>MEVPEIEKQIGINLYSTDTTGLGGQLRQEIEDFIVKEITNREEGEEGKYLIVELTKRDWDTHHLTRTLSRILQVSQKRISVAGTKDKRALTTQKISIFDTDASEIEKIHLKDIELKVLGRSRKSVELGDLWGNDFRITVRNIENSPEETEALLKKTTDEILAQGGVPNFFGIQRFGSVRPVTHLVGKAIVEGNFEKAALLYIAEPFPEEPEETKNARQFVKDTLDFKEGLKTYPLRLGHERAMMNHLIANPEDYSGSFRVLPQNLYRMFVHGYQSYIYNIILCRRIEAGIPLNRAVEGDIVCFRNEVGLPDSSKTEKVTSETVNAMNRLLKLGRAFITAPLPGYNTEFASGIPGEIENGVLKELGVSLEGFNIEKFPEMSSKGTRREVLLEVKP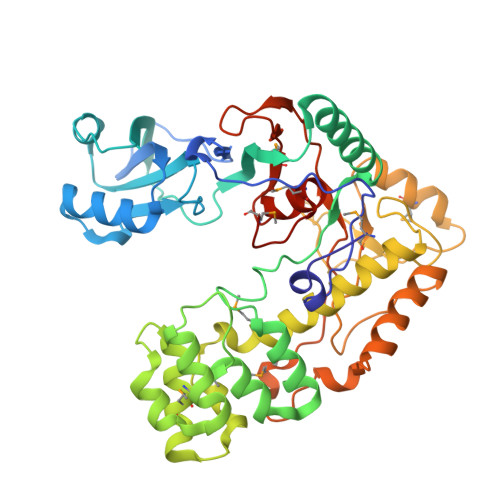KFEAGEDELNPGKSKAVLEFMLPKGSYATTVLREYMKVNPLQMSLEHHHHHH[2x]Cellvibrio japonicus is a saprotrophic bacterium which possesses the remarkable ability to grow in isolation using a variety of hemicellulosic polysaccharides as sole carbon sources. It produces a diverse collection of GHs, assembling enzyme systems that can degrade cellulose, xylans, mannans, and xyloglucans, among others. Effective xyloglucan-degrading GH systems (recently reviewed by Attia and Brumer) contain exo-acting glycosidases acting as debranching accessory enzymes and endo-acting enzymes (xyloglucanases) that generate short, branched β-(1,4)-glucan oligomers (xyloglucan oligosaccharides).18−23Exo-acting enzymes are expected to address each of the glycosidic linkages reported in xyloglucan branches, though the reported enzyme diversity falls short of reported branch diversity. The work presented here comprises the design and validation of trisaccharidic xyloglucan (“XyG”)-type cyclophellitol probes and their validation as bona fide, predictive tools for the identification of xyloglucanase activities and their discrimination from cellulase activities within a xyloglucan-elicited C. japonicus degradome.

Not having been previously functionally or structurally characterized in detail, we produced and purified Cel5B and Cel5C recombinantly in E. coli to assess further the correlation between probe reactivity and enzyme specificity. We found that Cel5B and Cel5C were both cellulases, efficiently degrading carboxymethylcellulose and mixed-linkage β-glucan. Cel5B showed only weak activity toward tamarind xyloglucan while Cel5C had weak activity toward carob galactomannan and no detectable xyloglucanase activity. To determine the molecular basis for the reactivity of ABP-XyG-Cy5 with CjCel5B but not CjCel5C, we crystallized both enzymes and solved their structures by molecular replacement in both unliganded and ABP-bound forms. Cel3A/B and Cel5C showed no change in expression under any condition tested, indicating that these are constitutively expressed.

>[3x]MDNAWQNTSGWWNAGDVPAFDKRQLSRQLPLIRVDGNRFVDEQGNVQIFRGVSISDPNKLAKDQHFNKKHFDVIRSWGTNVVRIPVHPSAWRERGVKGYLELLDQAITWNNELGMYTIIDWHSMGNLKSEMFQNSMYHTSKGETFDFWRRVSERYNGINSVAFYEIFNEPTVFSGRLGIVSWAEWKAINEEAITIIQAHNPNAISLVAGFNWAYDLREAAANPIERNNVAYVSHPYPQKVGAPYQANWERDFGFMADKYPVFATEIGYQLASDKGAHIPVIDDGSYGPRITDYFAKKGISWVAWVFDPDWSPQMIKSWDYEPTMQGEHFRKVMLKENKLEHHHHHH>[2x]SAKEKFTSLSPAEFFKRNPELAGFPNPARALYQTVRELIENSLDATDVHGILPNIKITIDLIDDARQIYKVNVVDNGIGIPPQEVPNAFGRVLYSSKYVNRQTRGMYGLGVKAAVLYSQMH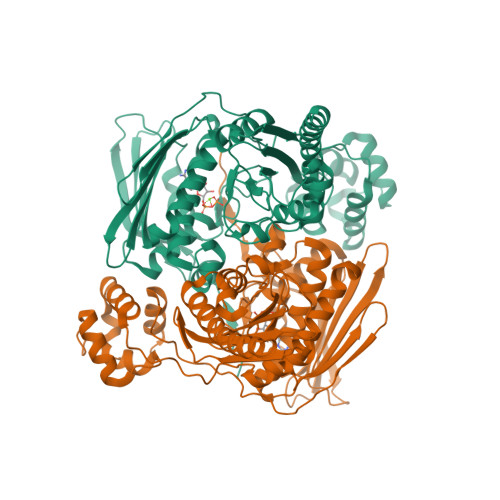QDKPIEIETSPVNSKRIYTFKLKIDINKNEPIIVERGSVENTRGFHGTSVAISIPGDWPKAKSRIYEYIKRTYIITPYAEFIFKDPEGNVTYYPRLTNKIPKPPQEVKPHPYGVDREEIKILINNLKRDYTIKEFLVNEFQSIGDTTADKILELAGLKPNKKVKNLTEEEITRLVETFKKYEDFRSPSADSLSVIGEDLIELGLKKIFNPDFAASITRKPKAYQGHPFIVEAGVAFGGSIPVGEEPIVLRYANKIPLIYDEKSDVIWKVVEELDWKRYGIESDQYQMVVMVHLCSTKIPYKSAGKESIAEVEDIEKEIKNALMEVARKLKQYLSEKRKEQEAKKKLLA>[4x]GGGGSMSTAEPAPDPTNPSTSGLAPTTNGIGSPPPTASAATKFSILTKFLRRKNQVHTTTAQQNEFMQKYMPNGNSNAVQPAATGGQPASSDGGSAIEVPPPKESYAVRIRKYLANYTQDPSTDNFYYWTCVVTVAYIYNLLFVIARQVFNDLIGPSSQSLCRFYNGTLNSTTQVECTYN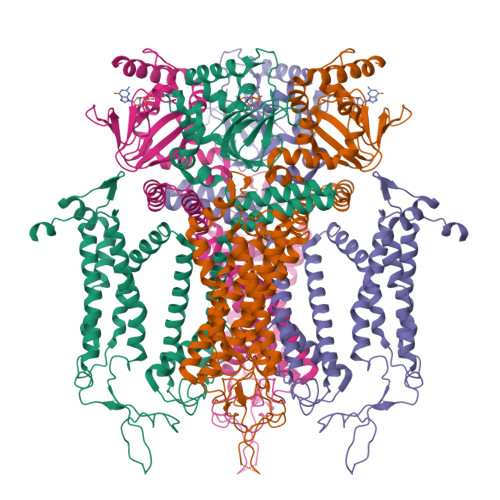MLTNMKEMPTYSQYPDLGWSKYWHFRMLWVFFDLLMDCVYLIDTFLNYRMGYMDQGLVVREAEKVTKAYWQSKQYRIDGISLIPLDYILGWPIPYINWRGLPILRLNRLIRYKRVRNCLERTETRSSMPNAFRVVVVVWYIVIIIHWNACLYFWISEWIGLGTDAWVYGHLNKQSLPDDITDTLLRRYVYSFYWSTLILTTIGEVPSPVRNIEYAFVTLDLMCGVLIFATIVGNVGSMISNMSAARTEFQNKMDGIKQYMELRKVSKQLEIRVIKWFDYLWTNKQSLSDQQVLKVLPDKLQAEIAMQVHFETLRKVRIFQDCEAGLLAELVLKLQLQVFSPGDFICKKGDIGREMYIVKRGRLQVVDDDGKKVFVTLQEGSVFGELSILNIAGSKNGNRRTANVRSVGYTDLFVLSKTDLWNALREYPDARKLLLAKGREILKKDNLLDENAPEEQKTVEEIAEHLNNAVKVLQTRMARLIVEHSSTEGKLMKRIEMLEKHLSRYKALARRQKTMHGVSIDGGDISTDGVDERVRPPRLRQTKTIDLPTGTESESLLK> L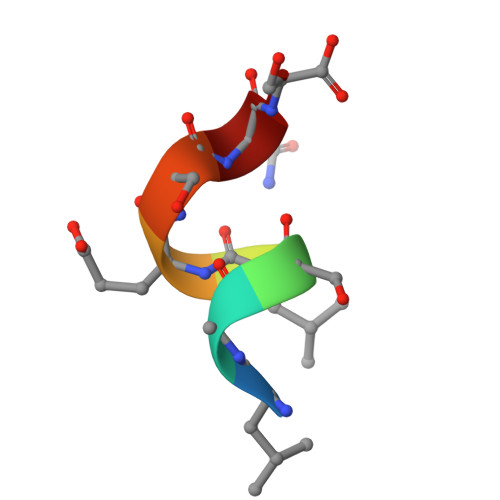ASLESQS>[2x]MAAAAPAETMNKSAAGAEVPE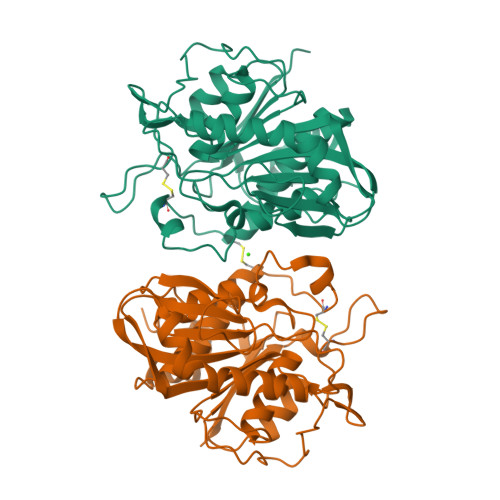AFTSVFQPGKLAVEAIQVDENAAPTPPIPVLIVAPKDAGTYPVAMLLHGFFLHNHFYEHLLRHVASHGFIIVAPQFSISIIPSGDAEDIAAAAKVADWLPDGLPSVLPKGVEPELSKLALAGHSRGGHTAFSLALGHAKTQLTFSALIGLDPVAGTGKSSQLQPKILTYEPSSFGMAMPVLVIGTGLGEEKKNIFFPPCAPKDVNHAEFYRECRPPCYYLVTKDYGHLDMLDDDAPKFITCVCKDGNGCKGKMRRCVAGIMVAFLNAALGEKDADLEAILRDPAVAPTTLDPVEHRVAENLYFQ> APVRSLNCTLRDSQQKSLVMSGPYELKALHLQGQDMEQQVVWSMSFVQGEESNDKIPVALGLKEKNLYLSCVLKDDKPTLQLESV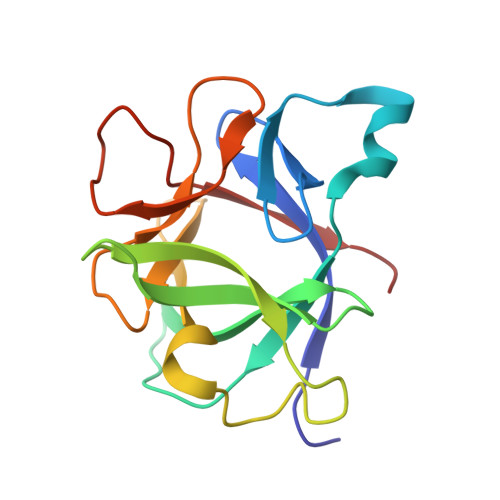DPKNYPKKKMEKRFVWNKIEINNKLEFESAQFPNWYISTSQAENMPVFLGGTKGGQDITDWTMQFVSS> GSMIRSTLSSWREYLTPITHKSTFLTTGQITPEEFVQAGDYLCHMFPTWKWNEESSDISYRDFLPKNKQFLIIRKVPCDKRAEQCVEVEGPDVIMKGFAE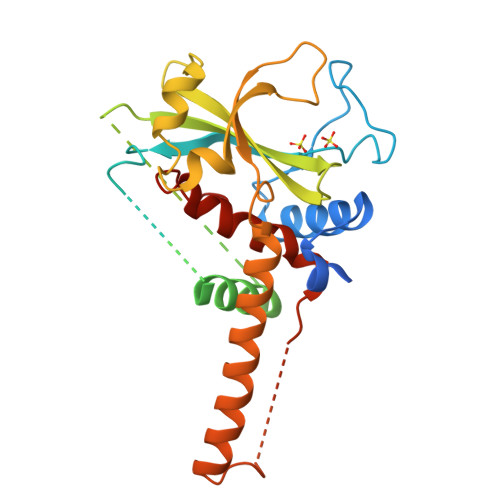DGDEDDVLEYIGSETEHVQSTPAGGTKDSSIDDIDELIQDMEIKEEDENDDTEEFNAKGGLAKDMAQERYYDLYIAYSTSYRVPKMYIVGFNSNGSPLSPEQMFEDISADYRTKTATIEKLPFYKNSVLSVSIHPCKHANVMKILLDKVRVVRQRRRKELQEEQELDGVGDWEDLQDDIDDSLRVDQYLIVFLKFITSVTPSIQHDYTMEGW>[2x]MAIPAFHPGELNVYSAPGDVADVSRALRLTGRRVMLVPTMGALHEGHLALVRAAKRVPGSVVVVSIFVNPMQFGAGGDLDAYPRTPDDDLAQLRAEGVEIAFTPTTAAMYPDGLRTTVQPGPLAAELEGGPRPTHFAGVLTVVLKLLQIVRPDRVFFGEKDYQQLVLIRQLVADFNLDVAVVGVPTVREADGLAMSSRNRYLDPAQRAAAVALSAALTA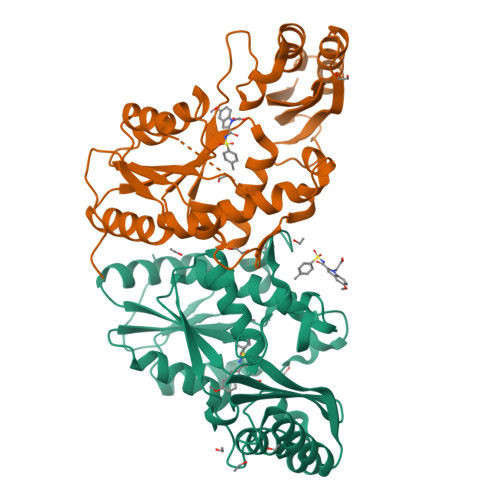AAHAATAGAQAALDAARAVLDAAPGVAVDYLELRDIGLGPMPLNGSGRLLVAARLGTTRLLDNIAIEIGTFAGTDRPDGYRAILESHWRN>[4x]SNAKDYQAGKNFTVIHSTVKQPPPLVEFFSFYCGPCYAFAERINVDTAIRKRLPDDMKLEKYHVSQMGPLGPALTEAWAVAQYAGVD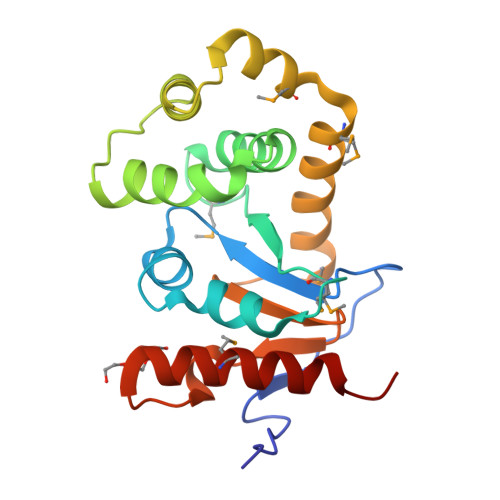GKVEKLLFEGLQVKRDIKTAADIVKVFNQLGITSEKYAEMQSNFMVKALIARQDNLVEKMKVHGTPSFYVSGKYHINNASLAQDDYDTYAEDMANLVLFLLNKPL> MVKLTPELINQSMQYINPVRERELDLRGYKIPQIENLGATLDQFDTIDLSDNDLRKLDNLPHLPRLKTLLLN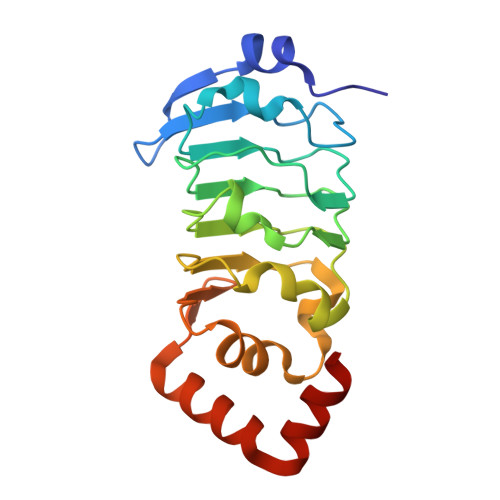NNRILRISEGLEEAVPNLGSIILTGNNLQELSDLEPLVGFTKLETISLLINPVSTKPNYREYMAYKFPQLRLLDFRKIKQKDRQAAQEFFRTKQGKDVLKEISR>[2x]GGVFPNVTNINSDKLLGGLLASGFDEDSCLSRYQSVHYRKPSPYKPSSYLISKLRNYEKLHKRCGPG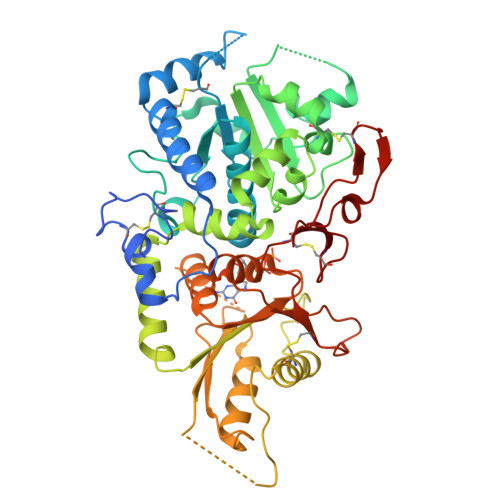TESYKKALKQLDQEHIDGDGECKYVVWISFSGLGNRILSLASVFLYALLTDRVLLVDRGKDMDDLFCEPFLGMSWLLPLDFPMTDQFDGLNQESSRCYGYMVKNQVIDTEGTLSHLYLHLVHDYGDHDKMFFCEGDQTFIGKVPWLIVKTDNYFVPSLWLIPGFDDELNKLFPQKATVFHHLGRYLFHPTNQVWGLVTRYYEAYLSHADEKIGIQVKVFDEDPGPFQHVMDQISSCTQKEKLLPEVDTLVERSRHVNTPKHKAVLVTSLNAGYAENLKSMYWEYPTSTGEIIGVHQPSQEGYQQTEKKMHNGKALAEMYLLSLTDNLVTSAWSTFGYVAQGLGGLKPWILYRPENRTTPDPSCGRAMSMEPCFHSPPFYDCKAKTGIDTGTLVPHVRHCEDISWGLKLV>MGDNIVLYYFDARGKAELIRLIFAYLGIEYTDKRFGVNGDAFVEFKNFKKEKDTPFEQVPILQIGDLILAQSQAIVRYLSKKYNICGESELNEFYADMIFCGVQDIHYKFNNTNLFKQNETTFLNEDLPKWSGYFEKLLKKNHTNNNNDKYYFVG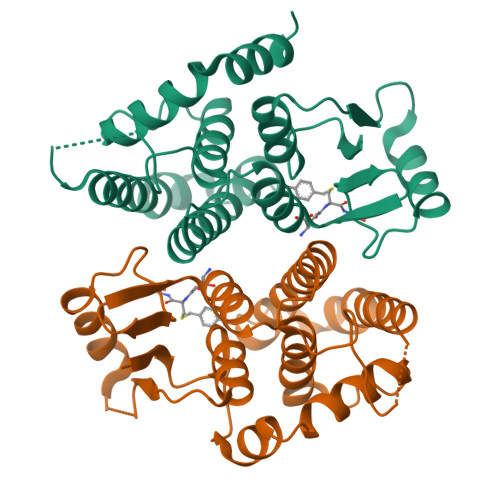NNLTYADLAVFNLYDDIETKYPSSLKNFPLLKAHNEFISNLPNIKNYITNRKESVY[2x]> GSTYHLDVVSAEQQMFSGLVEKIQVTGSEGELGIYPGHAPLLTAIKPGMIRIVKQHGHEEFIYLSGGILEVQPG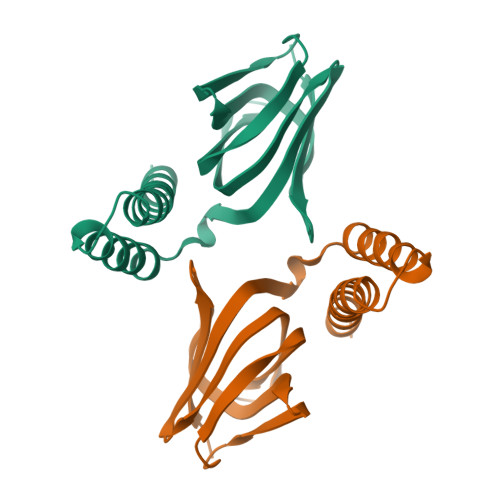NVTVLADTAIRGQDLDEARAMEAKRKAEEHISSSHGDVDYAQASAELAKAIAQLRVIELTKKAM>[2x]MHHHHHHSLLTEVETYVLSIVPSGPLKAEIAQRLEDVFAGKNTDLEVLMEWLKTRPILSPLTKGILGFVFTLTVPSERGLQRRRFVQNALNGNGDPNNMDKAVKLYRKLKREITFHGAKEIALSYSAGALASCMGLIYNRMGAVTTEVAFGLVCATCEQIADSQHRSHRQM

The matrix protein 1 (M1) of the influenza A virus is a 252-amino acid protein, comprised of an N-terminal domain (165 amino acids; N1–165-domain) and a C-terminal domain (87 amino acids; C166–252-domain), and plays an essential role in structural integrity, replication and budding of the virus. In the mature virion, M1 stabilizes the two major viral surface glycoproteins hemagglutinin (HA) and neuraminidase (NA) by forming a matrix layer underneath the lipid bilayer of the viral envelope. M1 also directly interacts with viral ribonucleoprotein (vRNP) consisting of viral RNA (vRNA), RNA polymerases and RNA-binding nucleoprotein (NP) and mediates the import of vRNP for vRNA synthesis in the nucleus of infected cells.

In the present study, we report a unique low-pH crystal structure of the M1 N1-165-domain of A/WSN/33 (H1N1) that shows a significant rotation (44–48°) of one of the monomers, resulting in a distinguishing dimer arrangement from previously reported low-pH M1 structures (vide infra). We have crystallized the truncated N1–165-domain of M1 using low salt and low pH (∼4.7) conditions in the space group P21 with unit-cell parameters a = 54.30, b = 37.35, c = 94.97 Å and β = 102.4°, and one dimer (monomers A and B) per asymmetric unit. Monomers A and B are related by a non-crystallographic 2-fold (perpendicular to H6) symmetry to form a dimer; placing the monomers in a face-to-face fashion that brings the two basic faces adjacent to each. The dimerization is maintained primarily by hydrophobic interactions between the symmetry-related helices H6 and to a lesser extent between helices H9 and loops L9, augmented by hydrogen-bond interactions involving Asn82, Arg101 and Asn133 of monomer A to Asn82, Asp94 and Gly88 of Monomer B. Monomer B shows significant disorder at the N-terminal domain containing residues 1–81 (H1–H5), and as a result residues 1, 17-19, 28–44, 72–74 could not be modelled. Figure 1 (D and E) shows analogous electron density maps of monomers A and B that illustrate a typical disorder in monomer B. Even the N-terminal domain residues that were included in the model show significantly higher than average B-factors of 92 Å2 compared to 67 Å2 for the C-terminal domain residues 82–156; similarly, the average B-factor for the entire B-chain was 78 Å2 compared to 38 Å2 for the entire A-chain. Importantly, helices H1–H5 seem to have unwound, with H2, H3 and H5 becoming unstructured. No other M1 structure shows such an extensive disorder, although residues 69-77 are known to be weak or disordered in other M1 structures. Although the unwinding of the N-terminal domain has not led to exposure of the H1 and H4 hydrophobic residues, this observation for the first time may indicate beginning of a domain rotation that exposes these residues as proposed by Sha & Luo.The norovirus genome contains three open reading frames (ORF1 to 3), where ORF1 encodes the nonstructural proteins, ORF2 encodes the capsid protein (VP1), and ORF3 encodes a minor structural protein (VP2). The S domain forms a scaffold surrounding the viral RNA, whereas the P domain contains the determinants of strain diversity and recognition of attachment factors. There is considerable antigenic drift among human noroviruses, and new genetic variants evolve every other year, which can result in new epidemics worldwide. It is well known that human noroviruses bind with various specificities to histo-blood group antigens (HBGAs), which are present in saliva, on the surface of epithelial cells, and in mucosal secretions. To elucidate the constraints on non-HBGA binders from a structural perspective, we determined the X-ray crystal structures of the capsid-protruding domains (P domains) of two GII.1 (HV and noro485) nonbinders and one GII.2 (SMV) HBGA nonbinder.

An earlier study by Huang et al. found that a GII.1 strain, termed Hawaii virus (HV), did not bind to HBGAs found in saliva and only weakly bound synthetic HBGA A and B types. Moreover, Harrington et al. observed that HV did not bind HBGAs in saliva or synthetic HBGAs, except for synthetic H type 1, which bound in a dose-dependent manner. HV, noro485, and SMV P domains diffracted to 1.86, 1.50, and 1.60 Å resolutions, respectively. In the HV and SMV P domains, we found two loop regions with disordered residues in the P2 subdomain, i.e., no discernible electron density, which suggested a certain degree of flexibility in these loops. In the HV P domain, Pro295 to Asp296 and Glu372 to Asp375 were disordered, while in the SMV P domain, residues Gln295 to Asp298 and Trp378 to Asp381 were disordered. The equivalent residues in the HV P domain were Cys345, Arg346, Asp375, and Gly438; in noro485, they were Cys345, Arg346, Asp375, and Gly438; and in SMV, they were Asn352, Arg353, Asp382, and Gly445. In the noro485 and SMV structures, Asp375 and Asp382, respectively, were pointing ~180° away from the fucose, whereas in the HV structure, Asp375 was missing because of the lack of electron density. In HV and SMV, loop B could not be modeled into the structures because of the lack of electron density. These data suggest that loop B might influence the stability of loop A, since loop B was missing from HV and partially missing from SMV. However, our new data indicate that Asp375 in HV, Asp375 in noro485, and Asp382 in SMV are unable to participate in the stabilization of the fucose moiety of HBGAs because of their flexibility or suboptimal orientation.

>GPGSKPFTLPILTIGELSNSRFPVPIDELYTSPNEGVIVQPQNGRSTLDGELLGTTQLVPSNICALRGRINAQVPDDHHQWNLQVTNTNGTPFDPTEDVPAPLGTPDFLANIYGVTSQRNPNNTCRAHDGVLATWSPKFTPKLGSVILGTWEESDLDLNQPTRFTPVGLFNTDHFDQWALPSYSGRLTLNMNLAPSVSPLFPGEQLLFFRSHIPLKGGTSDGAIDCLLPQEWIQHFYQESAPSPTDVALIRYTNPDTGRVLFEAKLHRQGFITVANSGSRPIVVPPNGYFRFDSWVNQFYSLAPM[2x]>AVVTAGVAGLGAIDAASATQKTNRASTVKGGFDYDVVVVGGGFAGATAARECGLQGYRTLLLEARSRLGGRTFTSRFAGQEIEFGGAWVHWLQPHVWAEMQRYGLGVVEDPLTNLDKTLIMYNDGSVESISPDEFGKNIRIAFEKLCHDAWEVFPRPHEPMFTERARELDKSSVLDRIKTLGLSRLQQAQINSYMALYAGETTDKFGLPGVLKLFACGGWNYDAFMDTETHYRIQGGTIGLINAMLTDSGAEVRMSVPVTAVEQVNGGVKIKTDDDEIITAGVVVMTVPLNTYKHIGFTPALSKGKQRFIKEGQLSKGAKLYVHVKQNLGRVFAFADEQQPLNWVQTHDYSDELGTILSITIARKETIDVNDRDAVTREVQKMFPGVEVLGTAAYDWTADPFSLGAWAAYGVGQLSRLKDLQAAEGRILFAGAETSNGWHANIDGAVESGLRAGREVKQLLSLEHHHHHH[2x]

The nicotine oxidoreductase NicA2 is a crucial enzyme for the first step of nicotine degradation in Pseudomonas putida S16 (DSM 28022). NicA2 from P. putida S16, 6HLNO and 6HDNO from A. nicotinovorans, and the nicotine oxidase NOX from Pseudomonas sp. strain HZN6 (21) belong to the family of flavin-dependent amine oxidases. In the NicA1- or NicA2-catalyzed reaction, flavin adenine dinucleotide (FAD) is required as a cofactor to couple the oxidation of nicotine with the reduction of oxygen to hydrogen peroxide. The structure of NicA2 comprises a FAD-binding domain (residues 49 to 129, 250 to 338, and 417 to 482) that harbors the cofactor FAD and a substrate-binding domain (residues 130 to 249 and 339 to 416) associated with the substrate nicotine.

Using this structure as a search model for molecular replacement, we then determined the crystal structure of the NicA2(21–482)–FAD–nicotine ternary complex at 2.25 Å resolution. In both structures, there are two complexes in each asymmetric unit. The nicotine molecule is bound midway between the S1 and S2 subdomains, with its pyrrolidine ring facing the FAD-binding domain. Unlike other, related structures, NicA2 does not have an associated diacyl glycerophospholipid, wraps its substrate more tightly, and has an intriguing exit passage in which nine bulky amino acid residues occlude the release of its toxic product, pseudooxynicotine (PN). Interestingly, the substrate nicotine is completely buried in the interior of NicA2 and is not accessible from the solvent when viewed from the substrate entry or product exit site. Only when the surface of NicA2 was set as transparent could the molecule nicotine be located deep inside the active-site pocket. When the product exit passage was investigated, it was found that this exit passage is blocked by many bulky residues, including W364, Y214, Y218, F355, F353, E249, F163, M246, and Y242. We hypothesized that the molecular deceleration via the severely restricted product exit tunnel strongly hinders the release of the reaction product PN from NicA2. Therefore, the substrate nicotine is deeply buried inside the active-site pocket of NicA2, and the exit passage is too occluded to allow the quick release of PN. Our results indicate that the passage in wild-type NicA2 effectively controls the rate of PN release and thus prevents its rapid intracellular accumulation.> MKIRQRQRFGRLELKRISGRGFKNDEEILIGNGTIQKIGIWDGEEEFHVRCGECRGILKKSQMRMEKLLINSAKKEDMKDLIILCMVFSQDTRMFQGVRGEINFLNRAGQLLSPMYQLQRYFLNRSNDLFDQWGYEESPKASELHGINELMNASD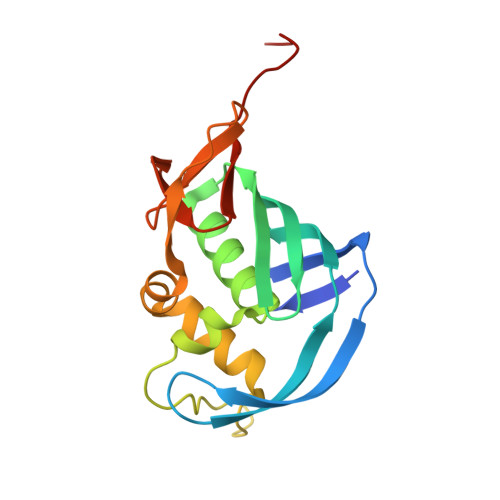YTLKGVVVTKNVDHHHHHH Btk is critical for the generation of calcium flux in response to receptor activation, because it activates phospholipase C-γ2 (PLC-γ2), which produces the second messengers diaceylglycerol (DAG) and inositol (1,4,5)-trisphosphate (IP3). Btk dysfunction is the cause of X-linked agammaglobulinemia, a severe disease of primary immunodeficiency. The Tec family kinases have a lipid-interaction module attached to the N terminus of a Src-like module (i.e., concatenation of an SH3 domain, an SH2 domain and a tyrosine kinase domain). The lipid-interaction module of the Tec kinases is an extended plekstrin homology (PH) domain fused to a Tec homology (TH) domain.

We expressed a ‘PH-TH-kinase’ construct of bovine Btk that contains the PH-TH module connected to the kinase domain by the 13-residue SH2-kinase linker. We replaced six residues in the activation loop of Btk with the corresponding ones in Itk, shown previously to stabilize the activation loop of the Btk kinase domain. The kinase domain is bound to the inhibitor CGI1746. The PH-TH module contacts the kinase N lobe. In Btk, the PH-kinase interface does not directly occlude the active site. The interface combines a set of hydrophobic contacts with a hydrogen-bond network. In particular, Tyr 134 at the C terminus of helix α2 of the PH-TH packs into a groove between Trp 395 at the linker-kinase junction and helix αC in the kinase N lobe. We expect these interactions to stabilize the inactive conformation of the kinase, by hindering the shift in helix αC that accompanies kinase activation. The IP4-binding site on the PH-TH module (the ‘canonical binding site’) is located ∼15 Å from the kinase-interacting surface of the PH-TH module. The structure of the PH-TH-kinase construct, in which no inositol phosphates are bound, resembles closely that of the liganded PH domain in the vicinity of the PH-kinase interface, consistent with the failure of IP4 to activate Btk.

> GMATVILESIFLKRSQQKKKTSPLNFKKRLFLLTVQKLSYYEYDFERGRRGSKKGSIDVEKITCVETVVPEKNPPPERQIPRRGEESSETEQISIIERFPYPFQVVYDEGPLYVFSPTEELRKRWIHQLKNVIRYNSDLVQKYHPCFWIDGQYLCCSQTAKNAMGCQILAAAPSTAGLGYGSWEIDPKDLTFLKELGTGQFGVVKYGKWRGQYDVAIKMIKEGSMSEDEFIEEAKVMMNLSHEKLVQLYGVCTKQRPIFIITEYMANGCLLNYLREMRHRFQTQQLLEMCKDVCEAMEYLESKQFLHRDLAARNCLVNDQGVVKVSDFGMTRYVLDDEYTSSTGSKFPVKWASPEVLMYSKFSSKSDIWAFGVLMWEIYSLGKMPYERFTNSETAEHIAQGLRLPRPHLASERVYAIMYSCWHEKADERPTFKILLSNILDVMDEE> GAEFMALPRLTGALRSFSNVTKQDNYNEEVADLKIKRSKLHEQVLDLGLTWKKIIKFLNEKLEKSKMQSINEDLKDILHAAKQIVGTDNGREAIESGAAFLFMTFHLKDSVGHKETKAIKQMFGPFPSSSATAACNATNRIISHFSQDDLTALVQMTEKEHGDRVFFGKNLAFSFDMHDLDHFDEL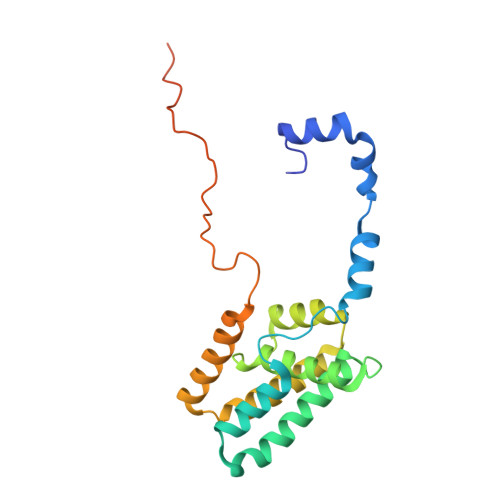PINGETQKTISLDYKKFLNEHLQEA> MNAHFANEVQYDLTRDPSSPASLIHVIISSECLAAAGVPLSALVRGRPDGGAAANFRVETQTRAHATGDCTPWRSAFAAYVPADAVGAILAPVIPAHPDLLPRVPSAGGLFVSLPVACDAQGVYDPYTVAALRLAWGPWATCARVLLFSYDELVPPNTRYAADGARLMRLCRHFCRYVARLGAAAPAAATEAAAHLSLGMGESGTPTPQASSVSGGAGPAVVGTPDPPISPEEQLTAPGGDTATAEDVSITQENEEILALVQRAVQDVTRRHPVRARPKHAASGVASGLRQGALVHQAVSGGALGASDAEAVLAGLEPPGGGRFASRG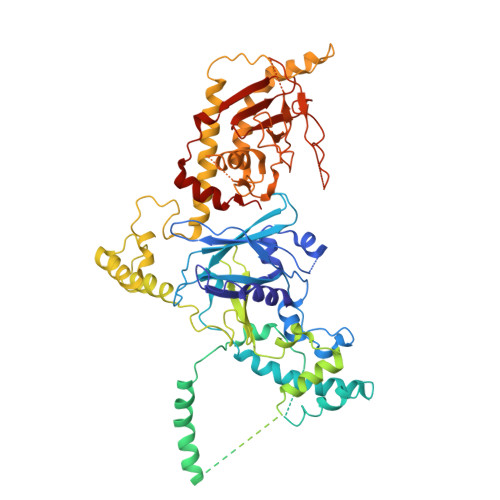GPRAAGEDVLNDVLTLVPGTAKPRSLVEWLDRGWEALAGGDRPDWLWSRRSISVVLRHHYGTKQRFVVVSYENSVAWGGRRARPPRLSSELATALTEACAAERVVRPHQLSPAAQTALLRRFPALEGPLRHPRPVLQPFDIAAEVAFVARIQIACLRALGHSIRAALQGGPRIFQRLRYDFGPHQSEWLGEVTRRFPVLLENLMRALEGTAPDAFFHTAYALAVLAHLGGQGGRGRRRRLVPLSDDIPARFADSDAHYAFDYYSTSGDTLRLTNRPIAVVIDGDVNGREQSKCRFMEGSPSTAPHRVCEQYLPGESYAYLCLGFNRRLCGLVVFPGGFAFTINTAAYLSLADPVARAVGLRFCRGAATGPGLVR Here, we choose lipase B from Candida antarctica (CALB), as the model enzyme, in which Asp187-His224-Ser105 is the catalytically active triad. Lipases function according to the classical Ser-His-Asp catalytic triad mechanism. In the present study we propose that the Ser → Cys conversion in lipases may lead to high activity by accurate manipulation of the local environment surrounding the hybrid Cys-His-Asp triad, enabled by laboratory evolution. We succeed in evolving cysteine-CALB mutants that are even more active than WT CALB.

Notably, variant QW10, which has the natural catalytic triad Ser-His-Asp restored and only differs from the best variant QW4 by the residue at position 105, displays lower activity than QW4 with the hybrid Cys-His-Asp triad (entry 11). In order to gain insight into the basis of increased activities of QW4 and QW10, the crystal structures of both enzymes were solved and refined to 1.85 and 1.88 Å resolution, respectively. Most residues in the structures of QW4 and QW10 have very similar conformations. The raised mobility of loop 137–150 in QW4 and QW10 enables ready entry of bulky substrates, which can be attributed to the introduction of the V149G mutation. In QW10 and WT, three or four H-bonds exist between S150/W155 and Q291, while in QW4 there are only two H-bonds between G149/W155 and Q291. The kinetic data shows, inter alia, that variants QW4 and QW10 are much more active for several substituted benzoates than WT and QW1. For QW10 and QW4, S105 and C105 remain in close proximity to the substrate carbonyl group, favorable for nucleophilic attack to occur. Extra space is created by the induced open conformation of the QW4 and QW10 variants compared with WT and QW2, which may also account for the high activities of the best mutants. An extensive QM/MM investigation showed that for the QW10 variant, the first step of the formation process of acyl-enzyme complexes works via a concerted mechanism in which the proton transfer from S105 to H224 occurs simultaneously with the nucleophilic attack to the carbonyl carbon atom of the substrate. The calculated reaction barrier is 10.56 kcal/mol and the reaction is exothermic, the energy of the tetrahedral product being 25.75 kcal/mol lower than that of the reactants.

>GAMALPSGSDPAFSQPKSVLDAGLTCQGASPSSVSKPILLVPGTGTTGPQSFDSNWIPLSAQLGYTPCWISPPPFMLNDTQVNTEYMVNAITTLYAGSGNNKLPVLTVSQGGLVAQWGLTFFPSIRSKVDRLMAFAPDYKGTVLAGPLDALAGSAPSVWQQTTGSALTTALRNAGGLTQIVPTTNLYSATDEIVQPQVSNSPLDSSYLFNGKNVQAQAVCGPLFVIDHAGSLTSQFSYVVGRSALRSTTGQARSADYGITDCNPLPANDLTPEQKVAAAALLAPYYAAIVAGPKQNCEPDLMPYARPFAVGKRTCSGIVTP[4x]> TGMSREEVESLIQEVLEVYPEKARKDRNKHLAVNDPAVTQSKKCIISNKKSQPGLMTIRGCAYAGSKGVVWGPIKDMIHISHGPVGCGQYSRAGRRNYYIGTTGVNAFVTMNFTSDFQEKDIVFGGDKKLAKLIDEVETLFPLNKGISVQSECPIGLIGDDIESVSK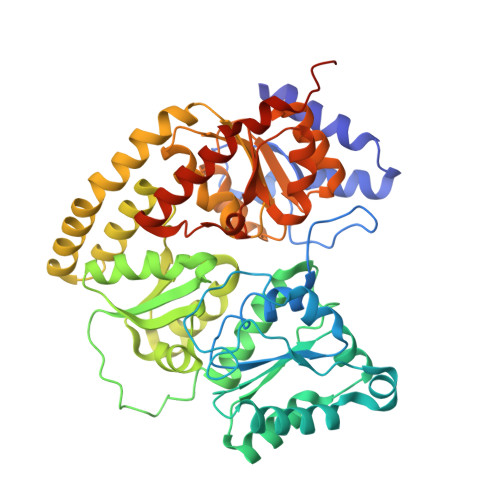VKGAELSKTIVPVRCEGFRGVSQSLGHHIANDAVRDWVLGKRDEDTTFASTPYDVAIIGDYNIGGDAWSSRILLEEMGLRCVAQWSGDGSISEIELTPKVKLNLVHCYRSMNYISRHMEEKYGIPWMEYNFFGPTKTIESLRAIAAKFDESIQKKCEEVIAKYKPEWEAVVAKYRPRLEGKRVMLYIGGLRPRHVIGAYEDLGMEVVGTGYEFAHNDDYDRTMKEMGDSTLLYDDVTGYEFEEFVKRIKPDLIGSGIKEKFIFQKMGIPFREMHSWDYSGPYHGFDGFAIFARDMDMTLNNPCWKKLQAPWEASEGAEKVAASA>MGHHHHHHAENLYFQGADPFESYNPEFFLYDIFLKFCLKYIDGEICHDLFLLLGKYNILPYDTSNDSIYACTNIKHLDFINPFGVAAGFDKNGVCIDSILKLGFSFIEIGTITPRGQTGNAKPRIFRDVESRSIINSCGFNNMGCDKVTENLILFRKRQEEDKLLSKHIVGVSIGKNKDTVNIVDDLKYCINKIGRYADYIAINVSSPNTPGLRDNQEAGKLKNIILSVKEEIDNLEK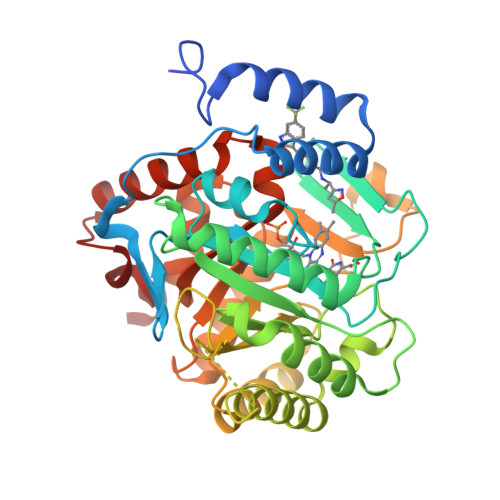NNIMNDEFLWFNTTKKKPLVFVKLAPDLNQEQKKEIADVLLETNIDGMIISNTTTQINDIKSFENKKGGVSGAKLKDISTKFICEMYNYTNKQIPIIASGGIFSGLDALEKIEAGASVCQLYSCLVFNGMKSAVQIKRELNHLLYQRGYYNLKEAIGRKHSKS[4x]>KDDFAKLEEQFDAKLGIFALDTGTNRTVAYRPDERFAFASTIKALTVGVLLQQKSIEDLNQRITYTRDDLVNYNPITEKHVDTGMTLKELADASLRYSDNAAQNLILKQIGGPESLKKELRKIGDEVTNPERFCPELNEVNPGETQDTSTARALVTSLRAFALEDKLPSEKRELLIDWMKRNTTGDALIRAGVPDGWEVADKTGAASYGTRNDIAIIWPPKGDPVVLAVLSSRDKKDAKYDDKLIAEATKVVMKALN[2x]

Here we report the crystal structure of a Class A β-lactamase PenP from Bacillus licheniformis 749/C with fluorescein conjugated at residue 166 after E166C mutation, both in apo form (PenP-E166Cf) and in covalent complex form with cefotaxime (PenP-E166Cf-cefotaxime), to illustrate its biosensing mechanism. Enzymes of this family deactivate β-lactam antibiotics by hydrolyzing the conserved β-lactam moiety in the antibiotics and rendering them ineffective to bind to their target proteins, the penicillin-binding proteins (PBPs), which are essential for bacterial cell wall synthesis and survival. For narrow-spectrum β-lactamases such as the PenP used in this study and the clinically significant TEM-1 or SHV-1 enzymes, Ω-loop is tightly packed onto the enzyme active site through hydrophobic and electrostatic interactions with residues lining the catalytic site, posing as steric hindrance for binding of second- or third-generation antibiotics with bulky side chains attached onto the β-lactam nucleus. Exploiting the proximity of Ω-loop to the antibiotic binding site and its structural flexibility, we have successfully converted a β-lactamase PenPC from Bacillus cereus 569/H into a biosensor for β-lactam antibiotics by mutating the catalytically critical residue Glu166 on the Ω-loop to cysteine and conjugating an environment-sensitive fluorescein molecule to its reactive side chain thiol group to form PenPC-E166Cf as reported in previous studies.

Cefotaxime was soaked into the PenP-E166Cf crystals by incubating the crystals in the reservoir solution with 0.01 M cefotaxime added for 20 minutes. The cefotaxime was clearly visible in fo-fc electron density map as covalently bonded through its carbonyl carbon atom C7 to the Oγ atom of Ser70, which represents the acylated ES* adduct. But we could not identify any electron density in either fo-fc or 2fo-fc map that would be accountable for fluorescein molecule around the location seen in PenP-E166Cf or anywhere nearby. Furthermore, the fo-fc map showed strong negative signal for a large segment of Ω-loop (residues 164 to 174) and the 2fo-fc map showed no electron density for this region at all, indicating this region became highly disordered upon acylation of cefotaxime. Based on these observations we did not include fluorescein molecule or the disordered region of Ω-loop in our final refined structure of PenP-E166Cf-cefotaxime. Fluorescein is seen as occupying a site that partially overlaps with the acylated cefotaxime; particularly the benzoic group of fluorescein molecule is in direct steric clash with the 7-amino substituent of cefotaxime. Thus the binding and acylation of cefotaxime to PenP would displace fluorescein from its original position to avoid steric clash. It is likely that the Ω-loop, in order to accommodate such displacement, loses its well-folded structure and becomes highly flexible.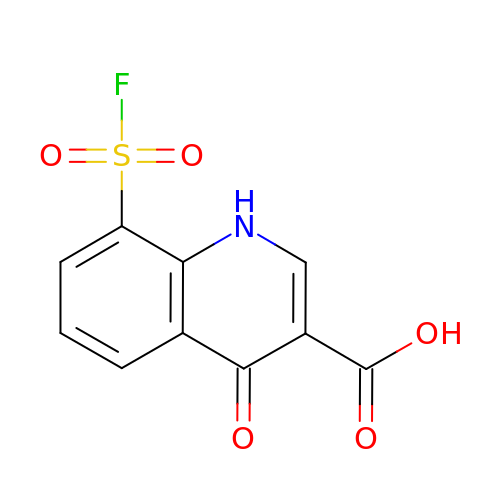8-(fluorosulfonyl)-4-oxo-1,4-dihydroquinoline-3-carboxylic acid | C10 H6 F N O5 S | HRNLMDOGOLJRKZ-UHFFFAOYSA-N>[2x]MGGSHHHHHHRSESTVTEELKEGIDAVYPSLVGTADSKAEGIKNYFKLSFTLPEEQKSRTVGSEAPLKDVAQALSSRARYELFTEKETANPAFNGEVIKRYKELMEHGEGIADILRSRLAKFLNTKDVGKRFAQGTEANRWVGGKLLNIVEQDGDTFKYNEQLLQTAVLAGLQWRLTATSNTAIKDAKDVAAITGIDQALLPEGLVEQFDTGMTLTEAVSSLAQKIESYWGLSRNPNAPLGYTKGIPTAMAAEILAAFVESTDVVENIVDMSEIDPDNKKTIGLYTITELDSFDPINSFPTAIEEAVLVNPTEKMFFGDDIPPVANTQLRNPAVRNTPEQKAALKAEQATEFYVHTPMVQFYETLGKDRILELMGAGTLNKELLNDNHAKSLEGKNRSVEDSYNQLFSVIEQVRAQSEDISTVPIHYAYNMTRVGRMQMLGKYNPQSAKLVREAILPTKATLDLSNQNNEDFSAFQLGLAQALDIKVHTMTREVMSDELTKLLEGNLKPAIDMMVEFNTTGSLPENAVDVLNTALGDRKSFVALMALMEYSRYLVAEDKSAFVTPLYVEADGVTNGPINAMMLMTGGLFTPDWIRNIAKGGLFIGSPNKTMNEHRSTADNNDLYQASTNALMESLGKLRSNYASNMPIQSQIDSLLSLMDLFLPDINLGENGALELKRGIAKNPLTITIYGSGARGIAGKLVSSVTDAIYERMSDVLKARAKDPNISAAMAMFGKQAASEAHAEELLARFLKDMETLTSTVPVKRKGVLELQSTGTGAKGKINPKTYTIKGEQLKALQENMLHFFVEPLRNGITQTVGESLVYSTEQLQKATQIQSVVLEDMFKQRVQEKLAEKAKDPTWKKGDFLT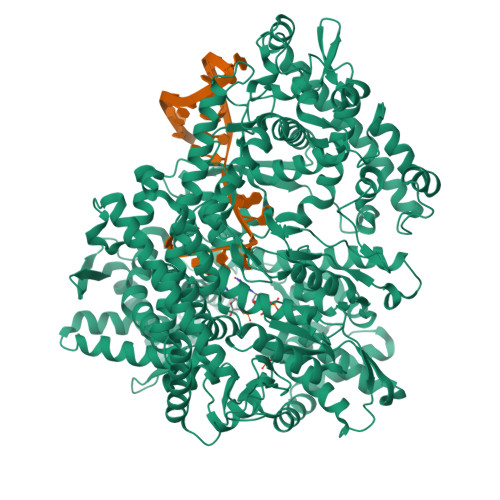QKELNDIQASLNNLAPMIETGSQTFYIAGSENAEVANQVLATNLDDRMRVPMSIYAPAQAGVAGIPFMTIGTGDGMMMQTLSTMKGAPKNTLKIFDGMNIGLNDITDASRKANEAVYTSWQGNPIKNVYESYAKFMKNVDFSKLSPEALEAIGKSALEYDQRENATVDDIANAASLIERNLRNIALGVDIRHKVLDKVNLSIDQMAAVGAPYQNNGKIDLSNMTPEQQADELNKLFREELEARKQKVAKA> MEKSQLESRVHLLEQQKEQLESSLQDALAKLKNRDAKQTVQK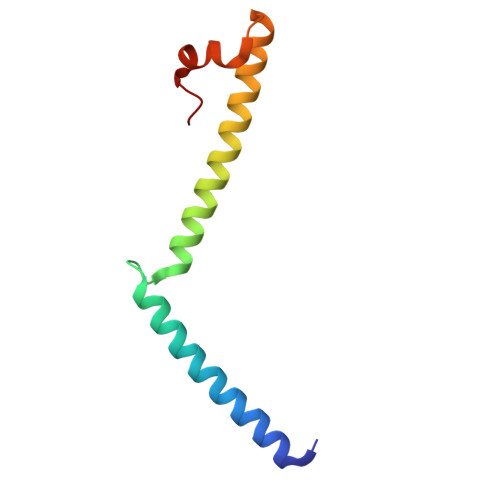HIDLLHTYNEIRDIALGMIGKVAEHEKCTSVELFDRFGVNGSE> SDAIKMFVGQVPRTWSEKDLRELFEQYGAVYEINVLRDRSQNPPQSKGCCFVTFYTRKAALEAQNALHNMKVLPGMHHP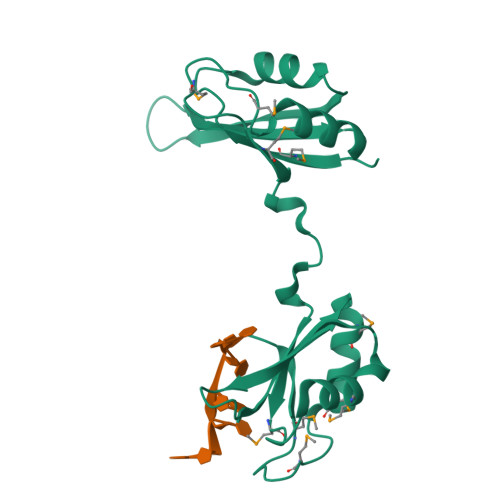IQMKPADSEKNNAVEDRKLFIGMISKKCTENDIRVMFSSFGQIEECRILRGPDGLSRGCAFVTFTTRAMAQTAIKAMHQAQTMEGCSSPMVVKFAD> MKEEQEVQATLESEEVDLNAGLHGNWTLENAKARLNQYFQKEK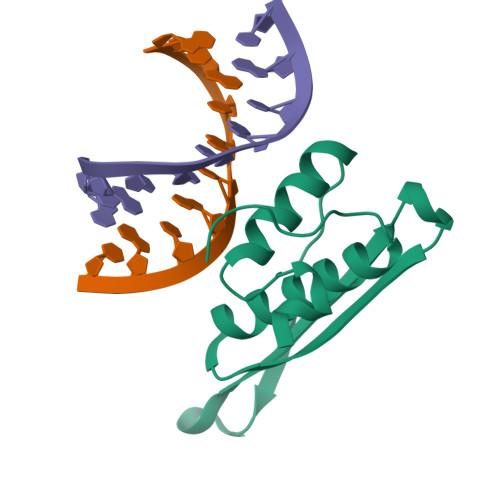IQGEYKYTQVGPDHNRSFIAEMTIYIKQLGRRIFAREHGSNKKLAAQSCALSLVRQLYHLGVVEAYSGLTK>[2x]DPVTLTLYNGQHAATGIAIAKAFQDKTGIQVKIRKGGDGQLASQITEEGARSP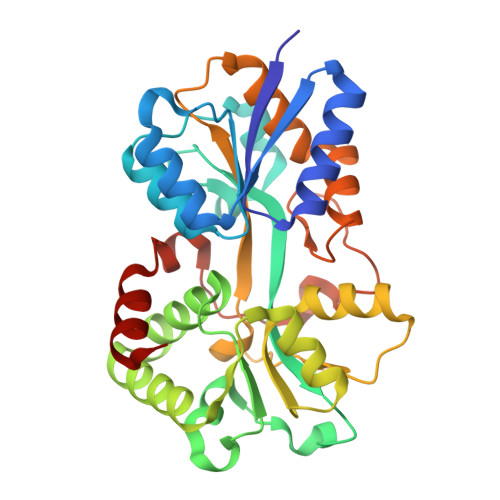ADVLYTEESPPLIRLASAGLLAKLEPETLALVEPEHAGGNGDWIGITARTRVLAYNPKKIDEKDLPKSLMDLSDPSWSGRFGFVPTSGAFLEQVAAVIKLKGQEEAEDWLTGLKAFGSIYTNNVTAMKAVENGEVDMALINNYYWYTLKKEKGELNSRLHYFGNQDPGALVTVSGAAVLKSSKHPREAQQFVAFMLSEEGQKAILSQSAEYPMRKGMQADPALKPFAELDPPKLTPADLGEASEALSLERDVGLN>MERLDIFGVPIDRVTMIQAVDILNNFLQENRLHIVATPNAEIVMMAQKDKEYMEILNNTDLNVPDGSGIVFASKVFKKPLPERVAGFDLMLEFIKGISSKGVKIYLLGAAAQVAE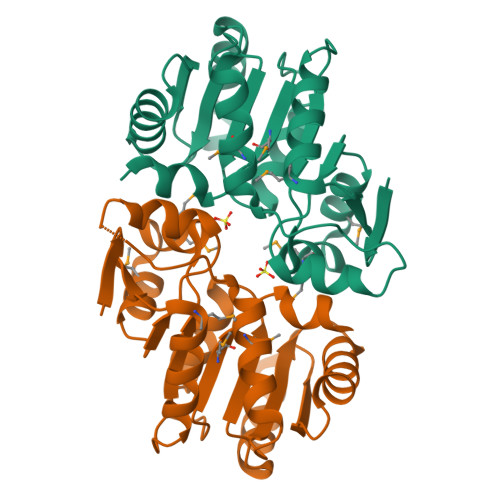QARANLEKLYPGVKIVGTHHGYFTEEEENKIIEEINNKGAEVLFVALGAPKQEKWIYKNKDKLKVKIAMGVGGSFDVIAG[8x]6-{[(1R,3R)-3-hydroxycyclopentyl]amino}pyridine-3-carboxamide | C11 H15 N3 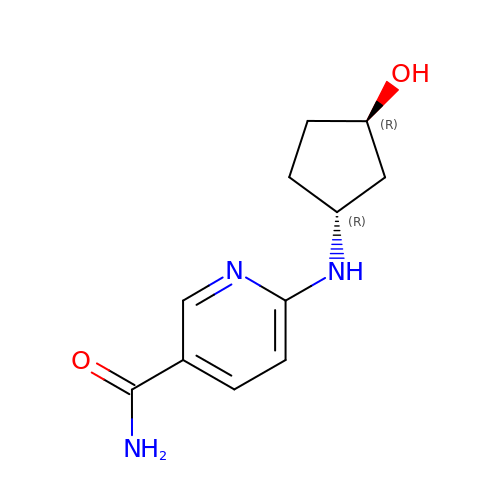O2 | PLJXPUZSPCVRPI-RKDXNWHRSA-N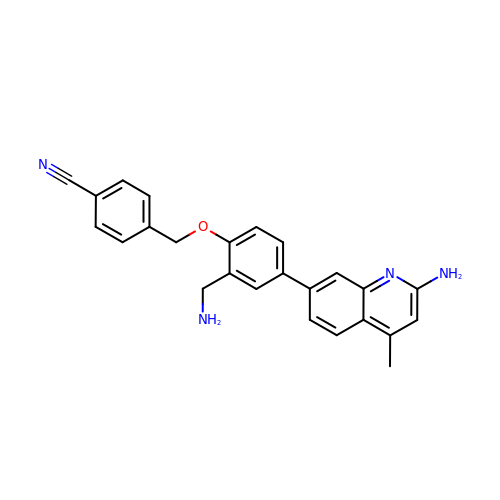4-{[2-(aminomethyl)-4-(2-amino-4-methylquinolin-7-yl)phenoxy]methyl}benzonitrile | C25 H22 N4 O | PKODNLRUHCVLDH-UHFFFAOYSA-N The I’m Not Dead Yet (INDY) protein in Drosophila melanogaster is a homodimeric plasma membrane transporter composed of 590 amino acids, belonging to the family of divalent anion–sodium symporters (DASS). INDY recognizes intermediates from the tricarboxylic acid cycle as substrates, with a preference for the dicarboxylate form of citrate at pH 6, and the anion exchanger inhibitor, DIDS (4,4′-diisothiocyano-2,2′-disulfonic acid stilbene), strongly inhibits its transport activity. Therefore, our biochemical characterization confirmed that INDY is a DIDS-sensitive H+/citrate symporter that predominantly recognizes citrate in its divalent form. Each protomer was divided into two domains: a central scaffold domain (TM 1–4 and 8–10), which plays an indispensable role in stable dimerization of the transporter, and a peripheral transport domain (HP1, HP2, TM 5–7, and TM 11–13) responsible for citrate binding and transport.

Apo-state structures of INDY were determined under two conditions: using nanodiscs at pH 6 and 8. The apo structures occurred in three conformations: (i) outward-open and (ii) inward-open conformations in which the substrate-binding site is exposed to the extracellular and intracellular sides, respectively, and (iii) an asymmetric conformation containing elements of both conformations. At pH 6, INDY exhibits two of these conformations, outward-open (43%) and asymmetric (57%). In the outward-open state, the substrate-binding site is positioned near the extracellular side at the membrane outer leaflet, and F119 adopts an upright orientation with respect to the membrane plane (left). This configuration allows the substrate to access the binding site from the extracellular side, while preventing its release inward (left). In a similar way, in the outward-open state, F119 in the downward position cannot be packed against TM 5b of the transport domain without encountering steric hindrance. The ability of INDY to adopt multiple configurations in the apo state highlights the intrinsic dynamics of the transporter independent of substrate binding.

>[2x]MATETTKMIYTPPPLDIKMEIEIGEQPQPPVKCSNFFANHWKGLVVFLVPLLCLPVMLLNEGAEFRCMYLLLVMAIFWVTEALPLYVTSMIPIVAFPIMGIMSSDQTCRLYFKDTLVMFMGGIMVALAVEYCNLHKRLALRVIQIVGCSPRRLHFGLIMVTMFLSMWISNAACTAMMCPIIQAVLEELQAQGVCKINHEPQYQIVGGNKKNNEDEPPYPTKITLCYYLGIAYASSLGGCGTIIGTATNLTFKGIYEARFKNSTEQMDFPTFMFYSVPSMLVYTLLTFVFLQWHFMGLWRPKSKEAQEVQRGREGADVAKKVIDQRYKDLGPMSIHEIQVMILFIFMVVMYFTRKPGIFLGWADLLNSKDIRNSMPTIFVVVMCFMLPANYAFLRYCTRRGGPVPTGPTPSLITWKFIQTKVPWGLVFLLGGGFALAEGSKQSGMAKLIGNALIGLKVLPNSVLLLVVILVAVFLTAFSSNVAIANIIIPVLAEMSLAIEIHPLYLILPAGLACSMAFHLPVSTPPNALVAGYANIRTKDMAIAGIGPTIITIITLFVFCQTWGLVVYPNLNSFPEWAQIYAAAALGNKTH>MTTLTARPEAITFDPQQSALIVVDMQNAYATPGGYLDLAGFDVSTTRPVIANIQTAVTAARAAGMLIIWFQNGWDEQYVEAGGPGSPNFHKSNALKTMRKQPQLQGKLLAKGSWDYQLVDELVPQPGDIVLPKPRYSGFFNTPLDSILRSRGIRHLVFTGIATNVSVESTLRDGFFLEYFGVVLEDATHQA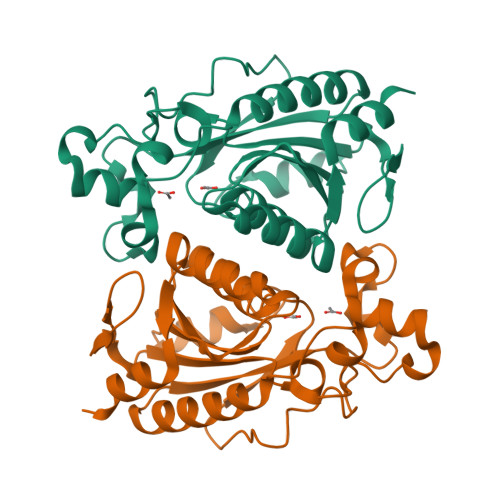GPKFAQKAALFNIETFFGWVSDVETFCDALSPTSFAHIA[16x]> GSHMPPNRPGITFEIGARLEALDWLQKWWPSRIEKIDYEEGKMLVHFERWSH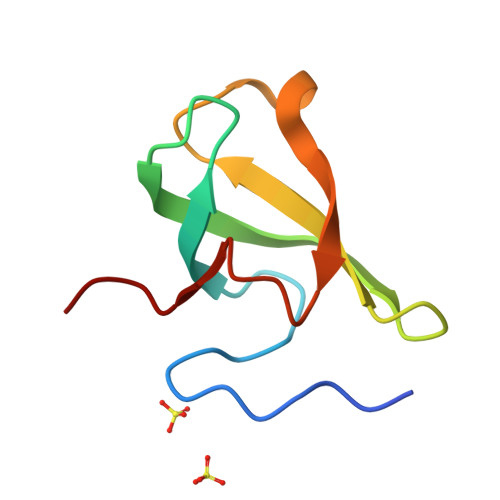RYDEWIYWDSNRLRPLER HJ resolvases are specific nucleases which nick the four arms of an HJ at the end of the recombination process. RecU is structurally different from the other HJ resolvases in the family, because of the presence of a central stalk region. RecU has a mushroom-like appearance with a cap (residues 34–55 and 90–199) and stalk sections (residues 56–89). Biochemical data showed that the stalk region of the RecU resolvase is essential for HJ recognition and distortion.

Therefore to gain insights into RecU DNA interactions, we crystallized an inactive mutant RecUD88N in complex with a palindromic 12 bp DNA. The asymmetric unit (ASU) of the crystal structure presented here consists of four RecU monomers (two dimers) and two dsDNA molecules. The two protein dimers are constituted by chains A plus C and B plus D and the two DNA duplexes are constituted by chains E plus F and G plus H. Each RecU monomer displays an α/β architecture and the structure of the protein is identical to the previous structure of unbound wildtype RecU with no indications at this resolution of any kind of large conformational change. The complete stalk region of RecU is visible in both dimers within the ASU of our complex structure. The 33 residue long NTR could be completely modeled for chain D. For chains A and C, the NTR could be modeled from residue 23 and 26 onwards, respectively, whereas for chain B we could not model any of the NTR residues. Duplexes fit along the concave surface of the mushroom cap of each monomer, which also contains the active site pockets. The stalk consists of a β-hairpin of class 12:12 in each monomer. The β-hairpins from the monomers cross over and extend toward the DNA duplex bound to the body of the other monomer in the dimer. Hence, the DNA binding pocket consists of a mushroom cap of one monomer and a stalk of a dimerizing partner. However, even at the low resolution, two hydrogen bonds are observed in all four monomers of the ASU: between the N atom of K165 and O1P of the nucleotide backbone; and between the OG atom of S166 and O2P of the nucleotide backbone.

>MIRYPNGKTFQPKHSVSSQNSQKRAPSYSNRGMTLEDDLNETNKYYLTNQIAVIHKKPTPVQIVNVHYPKRSAAVIKEAYFKQSSTTNYNGIYKGRYIDFEAKETKNKTSFPLQNFHDHQIEHMKQVKAQDGICFVIISAFDQVYFLEADKLFYFWDRKEKNGRKSIRKDELEETAYPISLGYAPRIDYISIIEQLYFS[4x]> ANIVGGIEYSINNASLCSVGFSVTRGATKGFVTAGHCGTVNATARIGGAVVGTFAARVFPGNDRAWVSLTSAQTLLPRVANGSSFVTVRGSTEAAVGAAVCHSGRTTGYQCGTITAKNVTANYAEGAVRGLTQSNACMGRGDSGGSWITSAGQAQGVMSGGNVQSNGNNCGIPASQRS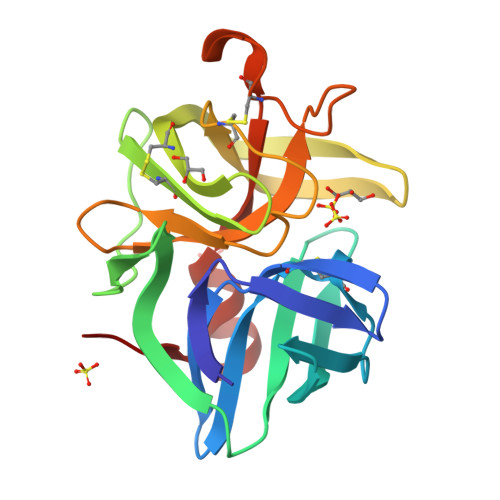SLFERLQPILSQYGLSLVTG>MPESVRYIKKKMHGEKLRKVEIEAIVRDIVDRKLRDIEISSFVTALEINGLDMDEIAALTIAMAETGDMLDIDRKPIMDVHSIGGVPGNKTNILVVPIVAAAGLTIPKTSSRAITSAAGTADVVEVFADVSFSLDEIKRIVEKVGACLVWGGALNLAPADDITIKAERALSIDPTGLMLASIMSKKYAMGSQYVLIDIPTGKGVKVETVEEARSLARDFIELGKRLGQYVEVAITYGGQPIGHTVGPALEAREALSALMTGKGPGSLIEKATGLAGILLEMGGVAPAGTGKKMAKEILESGKAWEKMKEIIEAQGGDPNIKPEEIPIGDKTYTFTAATSGYVTAI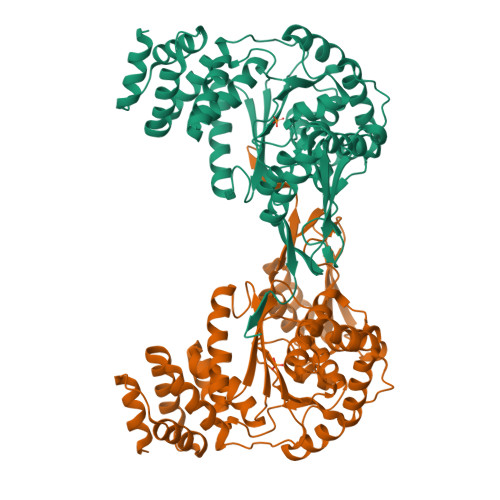DNRAITAIARAAGAPEDKGAGIELYVKVGEKVKEGDPLFTIHAEHEARLDQAIVLARRTEPIRIEGMVLQRIGNIGNSSSVDKLAAALEHHHHHH[2x]(3E)-4-hydroxybut-3-en-1-yl 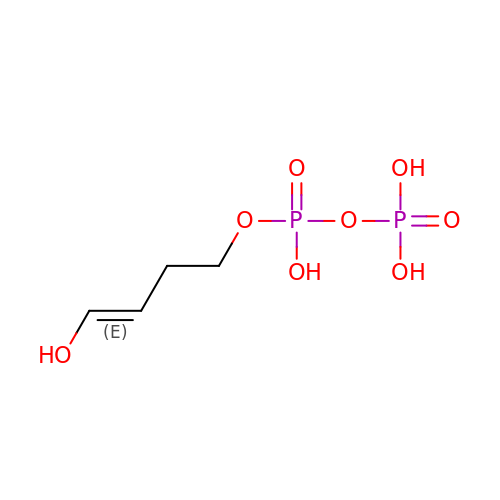trihydrogen diphosphate | C4 H10 O8 P2 | YCGPFMCUJHDYHD-HNQUOIGGSA-N>NSVLFPCKYASSGCEITLPHTEKAEHEELCEFRPYSCPCPGASCKWQGSLDAVMPHLMHQHKSITTLQGEDIVFLATDINLPGAVDWVMMQSCFGFHFMLVLEKQEKYDGHQQFFAIVQLIGTRKQAENFAYRLELNGHRRRLTWEATPRSIHEGIATAIMNSDCLVFDTS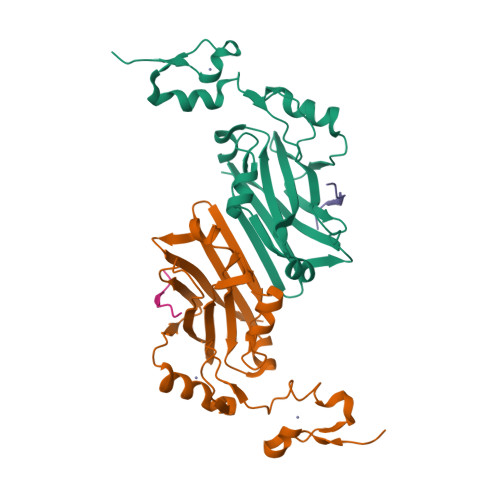IAQLFAENGNLGINVTISMC[4x];>LQQERTKLRPVAMVRPTVRVQPQL[4x]Escherichia coli possesses two acyl ornithine aminotransferases, one catabolic (AstC) and the other anabolic (ArgD), that participate in L-arginine metabolism. The arginine-succinyl transferase pathway of E. coli provides nitrogen for growth via a series of succinylated intermediates. In conclusion, the E. coli AstC protein, involved in arginine catabolism, is a PLP containing transaminase that is structurally similar to the related protein ArgD, which is the transaminase enzyme used in arginine synthesis. From the biochemical data, it appears that AstC and ArgD are biochemically similar, consistent with the ability of astC to complement an argD deletion. Both have comparable steady state kinetic values, with a strong preference for the acylated ornithine derivatives AO (AstC and ArgD) and SO (for AstC, at least) over ORN itself.

Crystals of holo-AstC diffracted to a higher resolution than the apo-protein (2.20 Å). Figures 4A and 4B show a dimer of holo-AstC, with PLP clearly bound in the cofactor site at the dimer interface. There is unambiguous density for the cofactor, and there is continuous density between Lys252 and the PLP, indicating that the expected aldimine had formed between the lysine residue and the PLP. There are four independent protomers in the asymmetric unit in the C2 crystal form, two full dimers, each protomer being almost equally resolved. In this case, the A–B and C–D dimer interfaces are also effectively equal, with a PISA analysis showing that the average surface area buried is 4752 Å2 (4764 Å2 for A–B and 4740 Å2 for C–D). The electron density for these residues is unambiguous in all of the PLP-bound structures of AstC and the A protomer of the PLP-free structure. In the AstC structures, the loop 277–282 ventures into the catalytic site of the neighboring protomer and makes important interactions to the cofactor (the distance from the Thr281 backbone nitrogen to an oxygen of PLP varies from 2.75 to 3.10 Å and the hydroxyl of Thr281 has a hydrogen bond of 2.5 to 3.0 Å to a phosphate oxygen). Dynamic light scattering indicates a hydrodynamic radius mean value 4.5 nm, indicative of a molecular weight of approximately 100 kDa (data not shown), suggesting that AstC is also a dimer in solution. SO, ORN and AO were docked into the active site of the structure with PLP covalently bound to Lys252, while αKG was docked into the non-covalently bound pyridoxamine phosphate structure.

>[4x]MSQPITRENFDEWMIPVYAPAPFIPVRGEGSRLWDQQGKEYIDFAGGIAVNALGHAHPELREALNEQASKFWHTGNGYTNEPVLRLAKKLIDATFADRVFFCNSGAEANEAALKLARKFAHDRYGSHKSGIVAFKNAFHGRTLFTVSAGGQPAYSQDFAPLPADIRHAAYNDINSASALIDDSTCAVIVEPIQGEGGVVPASNAFLQGLRELCNRHNALLIFDEVQTGVGRTGELYAYMHYGVTPDLLTTAKALGGGFPVGALLATEECARVMTVGTHGTTYGGNPLASAVAGKVLELINTPEMLNGVKQRHDWFVERLNTINHRYGLFSEVRGLGLLIGCVLNADYAGQAKQISQEAAKAGVMVLIAGGNVVRFAPALNVSEEEVTTGLDRFAAACEHFVSRGSS>MSALPELRELIASFVSEEPPEIRRIRTGTVPDLPGSYGQYFTAWDFSNSIVRDYAMNLYQLTRLATDESVS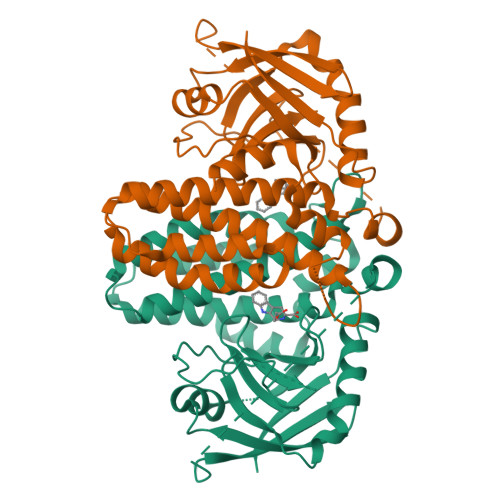VENLLTVFRTLDPIYSTFLGYNGFPVLAEYAQRVGQPAESRAELLDRLTTFTEYVNRLTAWSHHYFPWDLGGERYRYAAEEVAAQAAEAAAASPSVDSVDSLGDPSQRIPVRLTWQPLGVQVDAEIYADLNPQLATDVLKALPFTVLQDHAVVSGESMYAWAPLVSVAPTPVRERICDAPVGRLRFSQATGNKVIVQYGPTTETLSSPVLGKVVDSHADRLAEVGKAVWESTFSSKEPVWLTVERL[6x]> GHGHMHGRLKVKTSEEQAEAKRLEREQKLKLYQSATQAVFQKRQAGELDESVL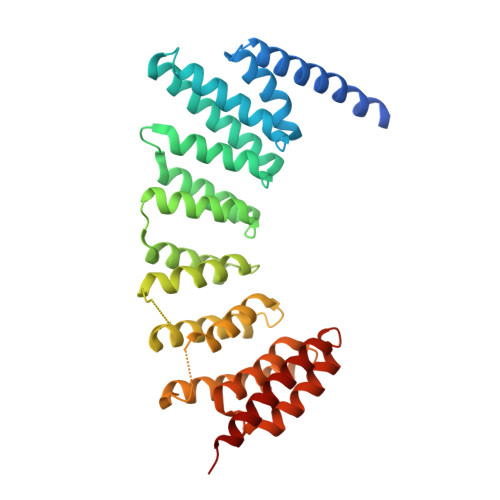ELTSQILGANPDFATLWNCRREVLQHLETEKSPEESAALVKAELGFLESCLRVNPKSYGTWHHRCWLLSRLPEPNWARELELCARFLEADERNFHCWDYRRFVAAQAAVAPAEELAFTDSLITRNFSNYSSWHYRSCLLPQLHPQPDSGPQGRLPENVLLKELELVQNAFFTDPNDQSAWFYHRWLLGAGSGRCELSVEKSTVLQSELESCKELQELEPENKWCLLTIILLMRALDPLLYEKETLQYFSTLKAVDPMRAAYLDDLRSKFLLENSVLKMEYA> SLAKRIIACLDVKDGRVVKGTNFENLRDSGDPVELGKFYSEIGIDELVFLDITASVEKRKTMLELVEKVAEQIDIPFTVGGGIHDFETASELILRGADKVSINTAAVENPSLITQIAQTFGSQAVVVAIDAKRVDGEFMVFTYSGKKNTGILLRDWVVEVEKRGAGEILLTSIDRDGTKSGYDTEMIRFVRPLTTLPIIASGGAGKMEHFLEAFLAGADAALAASVFHF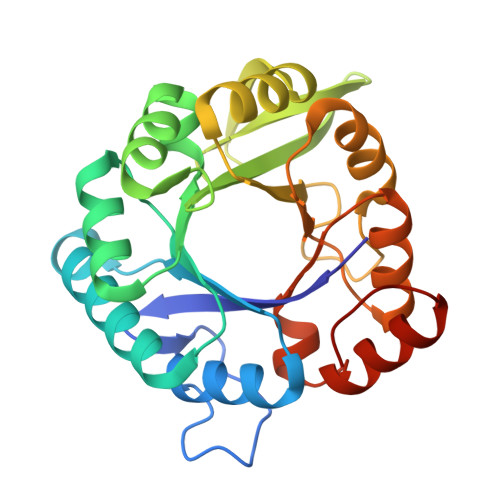REIDVRELKEYLKKHGVNVRLEGL>MLNQELELSLNMAFARAREHRHEFMTVEHLLLALLSNPSAREALEACSVDLVALRQELEAFIEQTTPVLPASEEERDTQPTLSFQRVLQRAVFHVQSSGRNEVTGANVLVAIFSEQESQAAYLLRKHEVSRLDVVNFISHGTRKDEPTQSSDPGSQPNSEEQAGGEERTENFTTNLNQLARVGGIDPLIGREKELERAIQVLCRRRKNNPLLVGESGVGKTAIAEGLAWRIVQGDVPEVMADCTIYSLDIGSLLAGTKYRGDFEKRFKALLKQLEQDTNSILFIDEIHTIIGAGAASGGQVDAANLIKPLLSSGKIRVIGSTTYQEFSNIFEKDRALARRFQKIDITEPSIEETVQIINGLKPKYEAHHDVRYTAKAVRAAVELAVKYINDRHLPDKAIDVIDEAGARARLMPVSKRKKTVNVADIESVVARIARIPEKSVSQSDRDTLKNLGDRLKMLVFGQDKAIEALTEAIKMARAGLGHEHKPVGSFLFAGPTGVGKTEVTVQLSKALGIELLRFDMSEYMERHTVSRLIGAPPGYVGFDQGGLLTDAVIKHPHAVLLLDEIEKAHPDVFNILLQVMDNGTLTDNNGRKADFRNVVLVMTTNAGVRETERKSIGLIHQDNSTDAMEEIKKIFTPEFRNRLDNIIWFDHLSTDVIHQVVDKFIVELQVQLDQKGVSLEVSQEARNWLAEKGYDRAMGARPMARVIQDNLKKPLANELLFGSLVDGGQVTVALDKEKNELTYGFQSAQKHKAEAAH[6x];>ALVPMVIEQTSRGERSFDIYSRLLKERVIFLTGQVEDHMANLIVAQMLFLEAENPEKDIYLYINSPGGVITAGMSIYDTMQFIKPDVSTICMGQAASMGAFLLTAGAKGKRFCLPNSRVMIHQPLGGYQGQATDIEIHAREILKVKGRMNELMALHTGQSLEQIERDTERDRFLSAPEAVEYGLVDSILTHRNRSHHHHHH[7x];> MGKTNDWLDFDQLAEEKVRDALKPPSMYKVILVNDDYTPMEFVIDVLQKFFSYDVERATQLMLAVHYQGKAICGVFTAEVAETKVAMVNKYARENEHPLLCTLEKA

ClpAP, a two-ring AAA+ protease, degrades N-end-rule proteins bound by the ClpS adaptor. AAA+ proteases, such as ClpAP, consist of a hexameric AAA+ unfoldase (for example, ClpA6) and a self-compartmentalized peptidase (for example, ClpP14). Each ClpA subunit has two AAA+ modules, called D1 and D2, that associate in the hexamer to form two stacked rings. Here we present high-resolution cryo-EM structures of Escherichia coli ClpAPS complexes, showing how ClpA pore loops interact with the ClpS N-terminal extension (NTE), which is normally intrinsically disordered.

In two classes, the NTE is bound by a spiral of pore-1 and pore-2 loops in a manner similar to substrate-polypeptide binding by many AAA+ unfoldases. For example, density for the ClpS NTE was present in both the ClpA D1 and D2 rings in classes I and II, but only in the D1 ring of class III. In classes I and II, residues 2–15 of the ClpS NTE were built into density in the D2 portion of the channel, but this NTE region was not visible in class III, presumably as a consequence of its conformational heterogeneity. The register of this ClpS peptide is very similar in each structure, with the C-terminal portion of the NTE (Pro24–Pro25–Ser26) near the top of the ClpA channel, and the N-terminal portion near the bottom of the channel in classes I and II. In classes II and III, the relative height of ClpA subunits was A (highest) > B > C > D > E > F (lowest), whereas in class-I, subunit B was higher than subunit A, resulting in a shallower spiral when aligned to the bottom of the IGL loop and the two flanking ClpP subunits. For example, the D2 GYVG pore-1 loops of all six ClpA subunits contacted the ClpS NTE in classes I and IIc, albeit the D2 pore-1 loop of subunit A had a lower buried surface area (BSA) in class I than in IIc. For instance, ADP is bound to the class-IIc D2 nucleotide sites in subunits E and F, but the GYVG loops from these domains contact the NTE. The presence of 11 engaged pore-1 loops (five D1 and six D2) probably contributes to the high affinity of ClpAPS•N-degron complexes assembled in ATPγS13. For example, in class IIc, the BSA values for the D1 KYR loops range from 63 to 196 Å2, the D1 pore-2 loops from 40 to 156 Å2 and the D2 GYVG pore-1 loops from 101 to 179 Å2. In contrast, the D2 pore-2 loops only weakly contact the NTE, as the BSA values of these interactions range from 20 to 74 Å2.> QKQQSERLGTEAIPKLLRSLSIPAMIGMFVMALYNVVDTIFISYAVGIEGVAGVTIAFPIMMIMMSMAGALGIGGASVISRRLGERRGEEANQVFGNILTVILVLSVIGFISAFTLLGPALQLFGATSVTQGYATDYLFPILLGSIFFFFAFAANNIIRSEGNATFAMVTMIVPAVLNILLDVLFIFGLNMGVLGASIATVIAQASVTGLVLRYFLTGKSTLSLHWSDLRMKGSVIKEVCLVGLPAFVQQSSASLMMIAINSMLLRFGSDFYVGVFGLVQRIMM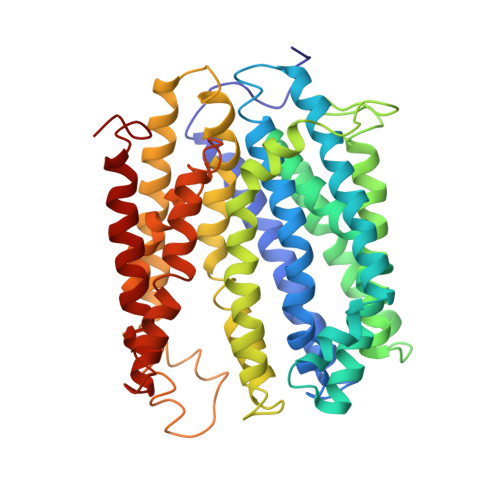FVMMPMMGIMQAMQPIVGYNYGAKQYSRLRETVMLGFKVATIFSIGIFALLMLFPEALLRVFTADREVIQAGVSAMHILFCVTFLIGAQIVAGGLYQSLGKPKQALILSLSRQIIFLIPLVLILPHIFGLSGVWWAFPIADVLSFILTVVLLYRDRNVFFLK> MVSLPRMVYPQPKVLTPCRKDVLVVTPWLAPIVWEGTFNIDILNEQFRLQNTT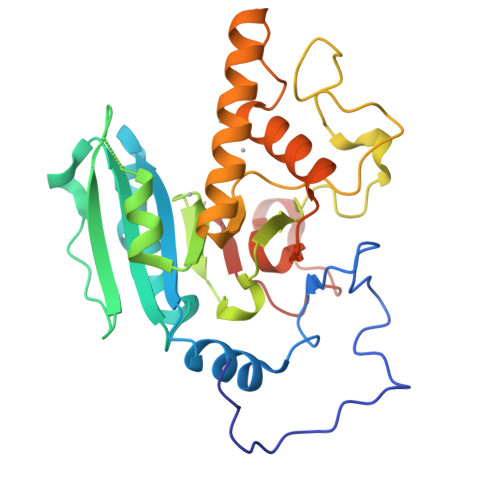IGLTVFAIKKYVAFLKLFLETAEKHFMVGHRVHYYVFTDQPAAVPRVTLGTGRQLSVLEVGAYKRWQDVSMRRMEMISDFCERRFLSEVDYLVCVDVDMEFRDHVGVEILTPLFGTLHPSFYGSSREAFTYERRPQSQAYIPKDEGDFYYMGAFFGGSVQEVQRLTRACHQAMMVDQANGIEAVWHDESHLNKYLLRHKPTKVLSPEYLWDQQLLGWPAVLRKLRFTAVPKNHQAVRNP> GVS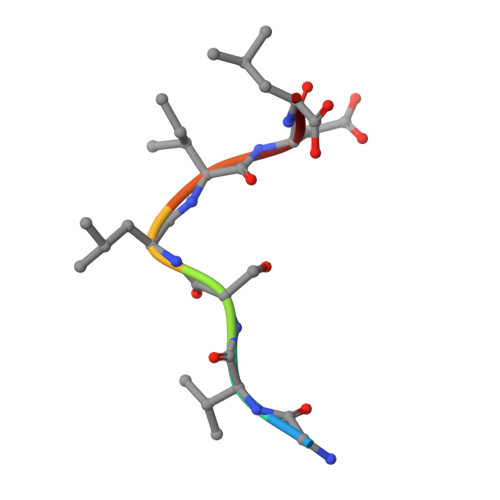LIDL> AGKNVNV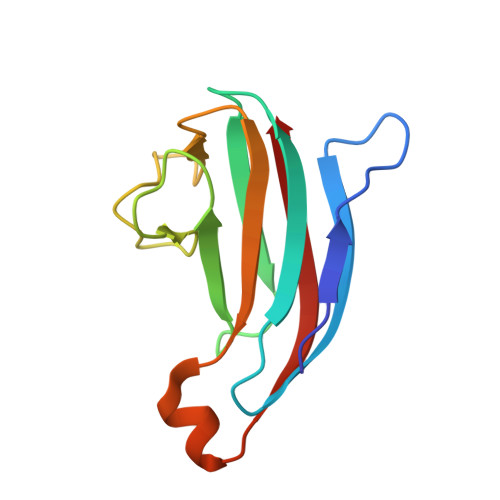EFRKGHSSAQYSGEIKGYDYDTYTFYAKKGQKVHVSISNEGADTYLFGPGIDDSVDLSRYSPELDSHGQYSLPASGKYELRVLQTRNDARKNKTKKYNVDIQIK>[5x]TVTYTNRVADARLGTFSQLLLQWKGSIYKLLYSEFLIFISLYFAISLVYRLILSESQRLMFEKLALYCNSYAELIPVSFVLGFYVSLVVSRWWAQYESIPWPDRIMNLVSCNVDGEDEYGRLLRRTLMRYSNLCSVLILRSVSTAVYKRFPSMEHVVRAGLMTPEEHKKFESLNSPHNKFWIPCVWFSNLAVKARNEGRIRDSVLLQGILNELNTLRSQCGRLYGYDWISIPLVYTQVVTVAVYSFFLACLIGRQFLDPEKAYPGHELDLFVPVFTFLQFFFYAGFLKVAEQLINPFGEDDDDFETNWLIDRNLQVSLMAVDEMHQDLPILEKDLYWNEPDPQEGEEF

BEST1-4 proteins are expressed in the plasma membrane and form Ca2+-activated Cl- channels by assembling as pentamers. The channel comprises five BEST1 subunits arranged symmetrically around a central ion pore that is ~95 Å long. The diameter of the pore varies along its length and contains two constrictions, the ‘neck’ and the ‘aperture’, both of which are lined by hydrophobic amino acids. To address these questions we determined a series of cryo-electron microscopy (cryo-EM) structures of chicken BEST1 with and without Ca2+ in activated, deactivated, and inactivated states that represent the major gating transitions of the channel.

W287 adopts one side chain rotamer to pack with F80 and F84 in the open conformation and a different side chain rotamer in the closed conformation that buttresses the space between adjacent neck helices. Because of its location and the conformational changes it undergoes, we hypothesized that W287 might propagate conformational changes in the Ca2+ clasp to the neck and thereby govern the conformation of the neck. We find that the W287F mutation (BEST1345 W287F) produces channels with dramatically altered gating. Whilst BEST1345 W287F retained normal Cl- versus K+ selectivity, the W287F mutation constitutively activates the channel, making it nearly insensitive to the presence or absence of Ca2+. Approximately, 80% of the Cl- current level through BEST1345 W287F is maintained when Ca2+ was chelated with EGTA, whereas currents through wild type BEST1 drop to zero. To understand the molecular basis of this behavior, we determined cryo-EM structures of BEST1345 W287F in the presence and absence of Ca2+ at 2.7 Å and 3.0 Å resolutions, respectively (Figure 4—figure supplements 1 and 2). In the presence of Ca2+, BEST1345 W287F adopts an open conformation that is essentially indistinguishable from the open conformation observed for BEST1345 (Cα RMSD = 0.2 Å). Unlike BEST1345, 3D classification of the BEST1345 W287F dataset did not reveal a closed conformation, which indicates that essentially all of the particles are in an open conformation and that the open state is preferential for this mutant. Thus, in accord with the electrophysiological recordings, the W287F mutation decouples Ca2+ binding from the conformational changes in the neck that are observed for the wild type channel. Modeling of the W287F mutation on a closed conformation of the channel introduces a void behind the neck, which we hypothesize energetically disfavors the closed conformation.HUSH is a complex of three proteins: transgene activation suppressor (TASOR), M-phase phosphoprotein 8 (MPP8), and Periphilin (PPHLN1, isoform 2). HUSH is a vertebrate-specific chromatin regulator that represses both exogenous and endogenous genetic elements. Here we show that TASOR is the central assembly platform of HUSH, providing binding sites for MPP8 and Periphilin. Structural and biochemical studies reveal that TASOR contains a catalytically inactive poly-ADP ribose polymerase (PARP) domain that is dispensable for assembly and chromatin targeting but critical for epigenetic regulation of target elements.

Bioinformatic analysis suggested that DUF3715 resembles a poly ADP-ribose polymerase (PARP) catalytic domain. Despite extensive trials, we could not induce the wild-type DUF3715 to crystallize. Hypothesizing that β6–β7 loop disorder precluded crystallization of the wild-type domain, we purified a variant with the Δ261–269 deletion. Validating our design, crystals were readily grown of native and SeMet-labeled samples, enabling X-ray structure determination of TASOR DUF3715 to a resolution of 2.0 Å by single-wavelength anomalous dispersion (SAD) phasing. In TASOR the key residues required for catalysis are even more degenerated than in ZAP or RCD1: all but one of them are replaced by hydrophobic amino acids. Based on our structure, TASOR therefore lacks the chemical functionality and physical space to bind the NAD+ cofactor. In particular, the loop connecting the final two strands (β8 and β9 in TASOR) spans 14 residues in TASOR (Tyr303–His316), compared to 5 residues in all annotated human PARP family members. In TASOR the extended β8–β9 loop has elevated B-factors in the crystal structure, and broad NMR peaks caused by fast T2 relaxation. We have identified that TASOR activity relies on an extended loop unique among the PARP family, and a single point mutation (Y305A) in this loop is sufficient to abolish transgene repression, endogenous LINE-1 restriction and genome-wide H3K9me3 deposition.

>KALFQPLTPGSREFEDVVNILHSSYLEPTSVTNFNYRRACLVHNELLEKEFTEKRRELKFDGRLDKELSESYAFLMVDRYQVQTICEKGLHVGQSKITILGSPSMGVYLSRYADLLQANPLDTGAMGDVVIFKIMKGKIKSIYDPMGVKSLDPTPKHECHVSKNANRITSLLAYRAYELTQYYFYEYGFDELRRRPRHVCPYAVVSFTYKDDIQ[2x]> MPKKNEAPASFEKALSELEQIVTRLES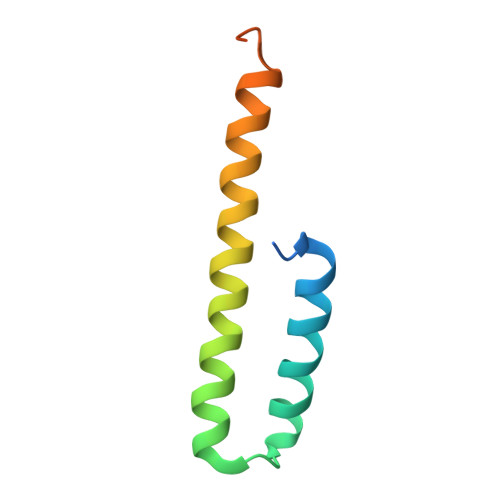GDLPLEEALNEFERGVQLARQGQAKLQQAEQRVQILLSDNEDASLTPFTPDNE>MGHHHHHHAENLYFQGHMHKVKLAAITCELPARSYENDDPVFAAVPDLSESWWQFWGVNRRGYFDPRNGENEFSLVVRAAERLLRSSDTAPDSVDMLICSASSPIMTDAGDVLPDLRGRLYPRMANVLSKQLGLSRALPLDSQMECASFLLNLRLAASMIRQGKAEKVLVVCSEYISNLLDFTSRTSTLFADGCAVALLTRGDDDSCDLLASAEHSDATFYEVATGRWRLPENPTGEAKPRLYFSLFSDGQNKMASFVPTNVPIAMRRALEKAGLGSDDIDYFVFHQPAPFLVKAWAEGIGARPEQYQLTMGDTGVMISVSIPYTLMTGLREGKIRPGDRIVMAGAATGWGFAAQVWQLGEVLVC[2x];>MLIQAVGVNLPPSYVCLEGPLGGERPRAQGDEMLMQRLLPAVREALDEAAVKPEEIDLIVGLALSPDHLIENRDIMAPKIGHPLQKVLGANRAHVFDLTDSSLARALYVVDTLASDQGYRNVLVVRGESSQGLEVDSESGFALADGALALLCRPTGKAAFRRGALGGD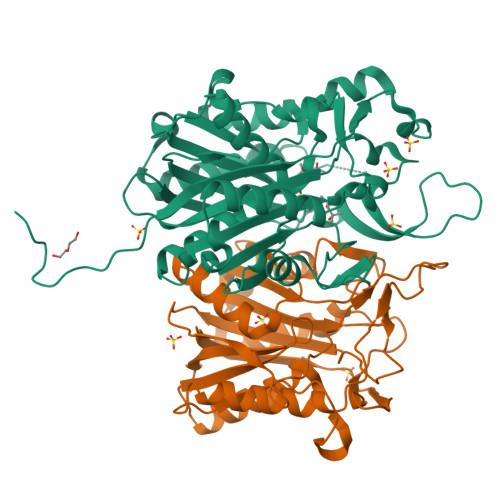PAQEWLPLSIPLNTDIRQVGDVKGHLNLPAQPGLPEAVRAGFTRLAGDFPQLNWVREEWFGQGRPDGRCLGPFELASQLRAAQRDRLDELLLISFDPFGMVVEGVTLELAGEAHA[2x]> PNIADKGSVFYHFSATSFDSVDGTRHYRVWTAVPNTTAPASGYPILYMLDGNAVMDRLDDELLKQLSEKTPPVIVAVGYQTNLPFDLNSRAYDYTPAAESRKTDLHSGRFSRKSGGSNNFRQLLETRIA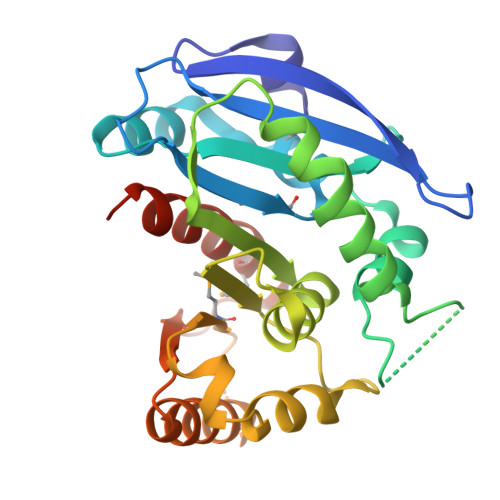PKVEQGLNIDRQRRGLWGHSYGGLFVLDSWLSSSYFRSYYSASPSLGRGYDALLSRVTAVEPLQFCTKHLAIMEGSATQGDNRETHAVGVLSKIHTTLTILKDKGVNAVFWDFPNLGHGPMFNASFRQALLDISGENANYTAGCHELSH>[4x]MNLKDKILGVAKELFIKNGYNATTTGEIVKLSESSKGNLYYHFKTKENLFLEILNIEQSKWQEQWKKEQIKAKTNREKFYLYNELSLTTEYYYP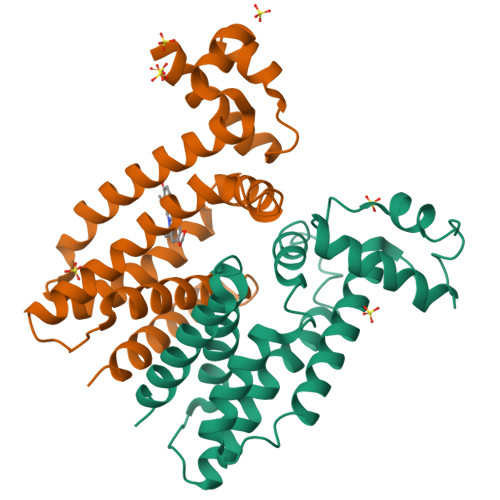LQNAIIEFYTEYYKTNSINEKMNKLENKYIDAYHVIFKEGNLNGEWSINDVNAVSKIAANAVNGIVTFTHEQNINERIKLMNKFSQIFLNGLSK1,3-thiazolidin-3-yl[(2S,4S)-4-{4-[2-(trifluoromethyl)quinolin-4-yl]piperazin-1-yl}pyrrolidin-2-yl]methanone | C22 H26 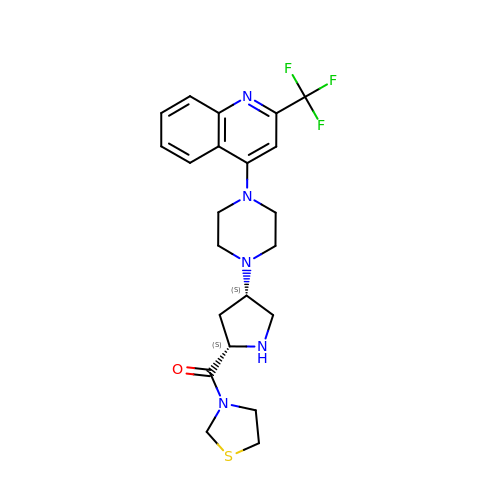F3 N5 O S | JWKZKADFQDTDIU-YJBOKZPZSA-N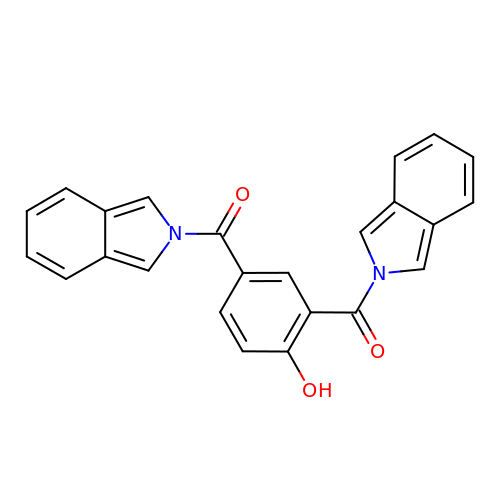(4-hydroxy-1,3-phenylene)bis[(2H-isoindol-2-yl)methanone] | C24 H16 N2 O3 | FQSLQNAXZJFWRX-UHFFFAOYSA-N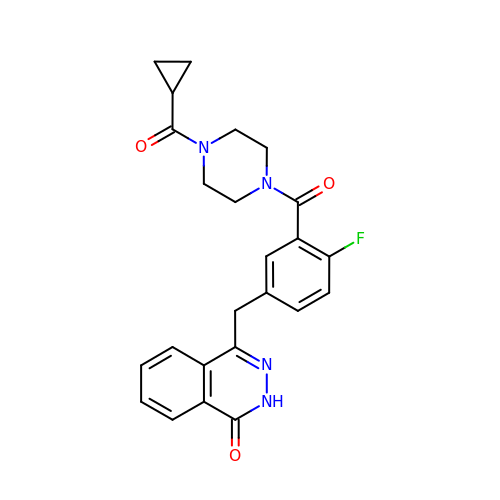4-(3-{[4-(cyclopropylcarbonyl)piperazin-1-yl]carbonyl}-4-fluorobenzyl)phthalazin-1(2H)-one | C24 H23 F N4 O3 | FDLYAMZZIXQODN-UHFFFAOYSA-N> ETGSAQQLNEDLRLHLLLNTSVTCNDGSPAGYYLKESRGSRRWLLFLEGGWYCFNRENCDSRYDTMRRLMSSRDWPRTRTGTGILSSQPEENPYWWNANMVFIPYCSSDVWSGASSKSEKNEYAFMGALIIQEVVRELLGRGLSGAKVLLLAGSAAGGTGVLLNVDRVAEQLEKLGYPAIQVRGLADSGWFLDNKQYRHTDCVDTITCAPTEAIRRGIRYWNGVVPERCRRQFQEGEEWNCFFGYKVYPTLRSPVFVVQWLFDEAQLTVDNVHLTGQPVQEGLRLYIQNLGRELRHTLKDVPASFAPACLSHEIIIRSHWTDVQVKGTSLPRALHCWDRSLHDSHKASKTPLKGCPVHLVDSCPWPHCNPSCPTGTKHHHHHH

The carboxylesterase Notum hydrolyzes a palmitoleate moiety from Wingless/Integrated(Wnt) ligands and deactivates Wnt signaling. Notum inhibitors can restore Wnt signaling which may be of therapeutic benefit for pathologies such as osteoporosis and Alzheimer’s disease. The overall structure maintained the characteristic apo Notum fold, with a α/β hydrolase core domain (β1-8 strands and αB, C, and F helices) and a moveable lid domain (αA, D, and E helices). Notum, like many other carboxylesterases, catalyzes reactions by forming a covalent acyl-enzyme intermediate.

To investigate the structural basis for this observation, we first soaked Notum crystals with 2 and determined a 1.4 Å resolution structure. The electron density for the acid head and indole ring electron densities were obvious, but there was little or no density for the butyric carbons, indicative of a degree of disorder. The electron density for the butyric carbons was restored when 2 was soaked into Notum S232A mutant crystals, consistent with the disorder arising from S232 sterically hindering optimal positioning of the acid form. Superposition of these two complexes with the 1 complex shows the interplay between nucleophile position and covalent or noncovalent inhibitor binding, with a shift in the S232 Cα of 0.6 Å between complexes involving 1 or 2. Our complex structures of the acid form 2 with Notum or its mutant demonstrate that the indole ring forms strong hydrophobic interactions with the Notum pocket residues and remains within the pocket.>[4x]MEKSQLESRVHLLEQQKEQLESSL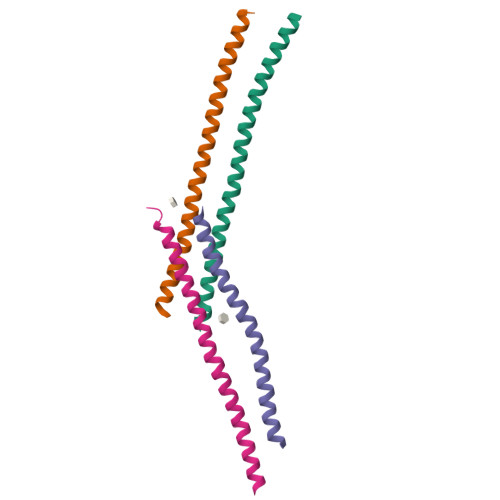QDALAKLKNRDAKQTVQKHIDLLHTYNEIRDIALGMIGKVAEHEKCTSVELFDRFGVNGSE> AVKLAPPTDVRSGYIRLV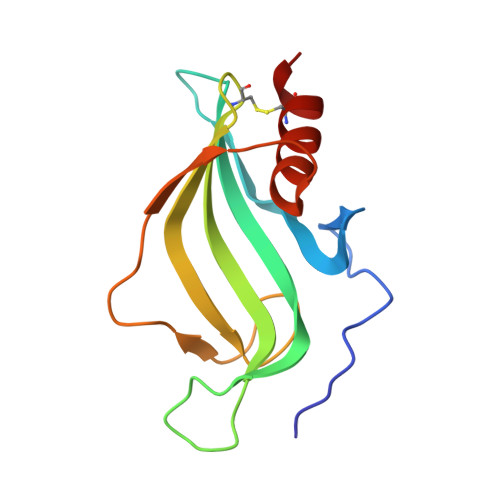KNVNYYIDSESIWVDNQEPQIVHFDAVVNLDKGLYVYPEPKRYARSVRQYKILNCANYHLTQVRTDFYDEFWGQGLRAAPKKQKKHTLSLTPDTTLYNAAQIICANYGK>SNAGMKAADFTYVTVHGDNSRMSRLKAQYTMLFFYDPDCSNCRKFEKLFAEIPAFVEMVENGTLRVLAIYPDENREEWATKAVYMPQGWIVGWNKAGDIRTRQLYDIRATPTIYLLDGRKRVILKDTSMEQLIDYLATQA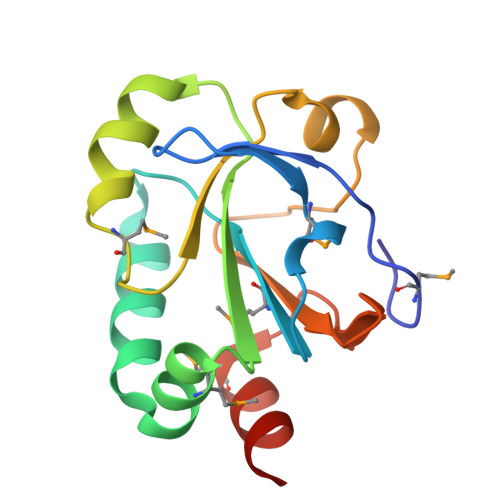GK[2x]ABC toxin complexes (Tcs) are a class of α-pore forming toxins (αPFTs) that consist of three subunits capable of assembling into a single protein apparatus with the ability to shuttle and translocate toxic peptides into target cells. The two TcAs termed Xn-XptA1 and Xn-XptA2 are the targeting components of each complex and display variations in insect specificity. The TcAs are the largest subunits of the complex and contain a translocation channel with hydrophobic loops at the end allowing for membrane permeation. Upon TcA binding and an environmental pH change, the complex undergoes a conformational change into an active state in which the translocation channel is exposed and pierces the target cell membrane.

To optimize the natural peptide shuttling and translocation mechanism of Xn-XptA2, our first strategy consisted of inserting the pharmacophore sequence of the TATE region of the DOTATATE peptide into the outermost loops of the NDs to alter the targeting potential of Xn-XptA2. We inserted the YWKT amino acids in between Threonine at position 1181 (T1181) and Proline at position 1183 (P1183) with the wt Aspartic Acid at position 1182 (D1182) replaced by the Threonine (T) in the YWKT sequence. The immunoreactive fraction was observed to be 2.8%, indicating no specific binding of Xn-XptA2 YWKT to SSTR2. To test whether the structural integrity of Xn-XptA2 YWKT was intact, we solved the structure to 4.3 Å resolution using cryo-EM single particle analysis (SPA). The biggest deviation in structure lies between G298 and P440. This stretch of 142 amino acids comprises RBD A on the periphery of the outer shell. The structural rearrangement of RBD A in Xn-XptA2 YWKT consists mainly of a significant loss in secondary structure in the form of β-sheets. In contrast, β-sheets in the Xn-XptA2 YWKT RBD A are only observed at positions G328-V335 and I433-P440 with the former regions of β-sheets rearranging into loops. RBD A is ~130 angstroms and 742 residues away from the outer loops of the ND at the YWKT insertion site (P440-T1181), indicating that disruption of these outer loops has an allosteric effect on upstream domains. Comparatively, in the Xn-XptA2 YWKT structure, the narrowest constriction point in the pore has a maximum radius of 4.6 Å and is also compressed by four amino acids from two separate protomers: D518 (Chain A), Q152 (Chain E), Q294 (Chain A), and K291 (Chain A).

>MYSTAVLLNKISPTRDGQTMTLADLQYLSFSELRKIFDDQLSWGEARHLYHETIEQKKNNRLLEARIFTRANPQLSGAIRLGIERDSVSRSYDEMFGARSSSFVKPGSVASMFSPAGYLTELYREAKDLHFSSSAYHLDNRRPDLADLTLSQSNMDTEISTLTLSNELLLEHITRKTGGDSDALMESLSTYRQAIDTPYHQPYETIRQVIMTHDSTLSALSRNPEVMGQAEGASLLAILANISPELYNILTEEITEKNADALFAQNFSENITPENFASQSWIAKYYGLELSEVQKYLGMLQNGYSDSTSAYVDNISTGLVVNNESKLEAYKITRVKTDDYDKNINYFDLMYEGNNQFFIRANFKVSREFGATLRKNAGPSGIVGSLSGPLIANTNFKSNYLSNISDSEYKNGVKIYAYRYTSSTSATNQGGGIFTFESYPLTIFALKLNKAIRLCLTSGLSPNELQTIVRSDNAQGIINDSVLTKVFYTLFYSHRYALSFDDAQVLNGSVINQYADDDSVSHFNRLFNTPPLKGKIFEADGNTVSIDPDEEQSTFARSALMRGLGVNSGELYQLGKLAGVLDAQNTITLSVFVISSLYRLTLLARVHQLTVNELCMLYGLSPFNGKTTASLSSGELPRLVIWLYQVTQWLTEAEITTEAIWLLCTPEFSGNISPEISNLLNNLRPSISEDMAQSHNRELQAEILAPFIAATLHLASPDMARYILLWTDNLRPGGLDIAGFMTLVLKESLNANETTQLVQFCHVMAQLSLSVQTLRLSEAELSVLVISGFAVLGAKNQPAGQHNIDTLFSLYRFHQWINGLGNPGSDTLDMLRQQTLTADRLASVMGLDISMVTQAMVSAGVNQLQCWQDINTVLQWIDVASALHTMPSVIRTLVNIRYVTALNKAESNLPSWDEWQTLAENMEAGLSTQQAQTLADYTAERLSSVLCNWFLANIQPEGVSLHSRDDLYSYFLIDNQVSSAIKTTRLAEAIAGIQLYINRALNRIEPNARADVSTRQFFTDWTVNNRYSTWGGVSRLVYYPENYIDPTQRIGQTRMMDELLENISQSKLSRDTVEDAFKTYLTRFETVADLKVVSAYHDNVNSNTGLTWFVGQTRENLPEYYWRNVDISRMQAGELAANAWKEWTKIDTAVNPYKDAIRPVIFRERLHLIWVEKEEVAKNGTYWKTPVETYDRFTLKLAFLRHDGSWSAPWSYDITTQVEAVTDKKPDTERLALAASGFQGEDTLLVFVYKTGKSYSDFGGSNKNVAGMTIYGDGSFKKMENTALSRYSQLKNTFDIIHTQGNDLVRKASYRFAQDFEVPASLNMGSAIGDDSLTVMENGNIPQITSKYSSDNLAITLHNAAFTVRYDGSGNVIRNKQISAMKLTGVDGKSQYGNAFIIANTVKHYGGYSDLGGPITVYNKTKNYIASVQGHLMNADYTRRLILTPVENNYYARLFEFPFSPNTILNTVFTVGSNKTSDFKKCSYAVDGNNSQGFQIFSSYQSSGWLDIDTGINNTDIKITVMAGSKTHTFTASDHIASLPANSFDAMPYTFKPLEIDASSLAFTNNIAPLDIVFETKAKDGRVLGKIKQTLSVKRVNYNPEDILFLRETHSGAQYMQLGVYRIRLNTLLASQLVSRANTGIDTILTMETQRLPEPPLGEGFFANFVLPKYDPAEHGDERWFKIHIGNVGGNTGRQPYYSGMLSDTSETSMTLFVPYAEGYYMHEGVRLGVGYQKITYDNTWESAFFYFDETKQQFVLINDADHDSGMTQQGIVKNIKKYKGFLNVSIATGYSAPMDFNSASALYYWELFYYTPMMCFQRLLQEKQFDEATQWINYVYNPAGYIVNGEIAPWIWNCRPLEETTSWNANPLDAIDPDAVAQNDPMHYKIATFMRLLDQLILRGDMAYRELTRDALNEAKMWYVRTLELLGDEPEDYGSQQWAAPSLSGAASQTVQAAYQQDLTMLGRGGVSKNLRTANSLVGLFLPEYNPALTDYWQTLRLRLFNLRHNLSIDGQPLSLAIYAEPTDPKALLTSMVQASQGGSAVLPGTLSLYRFPVMLERTRNLVAQLTQFGTSLLSMAEHDDADELTTLLLQQGMELATQSIRIQQRTVDEVDADIAVLAESRRSAQNRLEKYQQLYDEDINHGEQRAMSLLDAAAGQSLAGQVLSIAEGVADLVPNVFGLACGGSRWGAALRASASVMSLSATASQYSADKISRSEAYRRRRQEWEIQRDNADGEVKQMDAQLESLKIRREAAQMQVEYQETQQAHTQAQLELLQRKFTNKALYSWMRGKLSAIYYQFFDLTQSFCLMAQEALRRELTDNGVTFIRGGAWNGTTAGLMAGETLLLNLAEMEKVWLERDERALEVTRTVSLAQFYQALSSDNFNLTEKLTQFLREGKGNVGASGNELKLSNRQIEASVRLSDLKIFSDYPESLGNTRQLKQVSVTLPALVGPYEDIRAVLNYGGSIVMPRGCSAIALSHGVNDSGQFMLDFNDSRYLPFEGISVNDSGSLTLSFPDATDRQKALLESLSDIILHIRYTIR[5x]>[12x]MKEPRYLVPGDYMADPAAHVFNDKLYIYPSHDWESGIPENDNGDHFNMKDYHVFSMDDVEQGEVTDHGVVLRTEDIPWAGRQLWDSDVAFRNGKYYMYFPLKDQNDIFRIGVAISDRPEGPFIPQENPIKGSYSMDPCIWPDKDGEYYMYFGGLWGGQLQRYRNNKALECALLPEGDEPALCPKVVRLREDMLEFAEEPRDLMILDEKGKLLSAGDTKRRF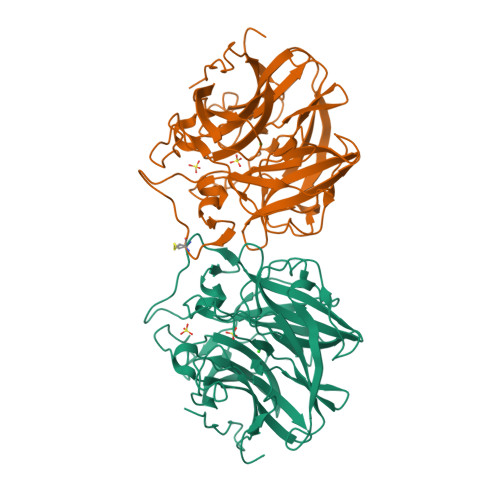FEASWMHYYNGKYYFSYSTGDTHLICYATGDNPYGPFTYRGVILTPVVGWTTHHSIVEFKGKWYLFHHDCVPSKGKTWLRSLKVAELKYNPDGSIQPIKGTAE>[2x]GSMAEPLKEEDGEDGSAEPPGPVKAEPAHTAASVAAKN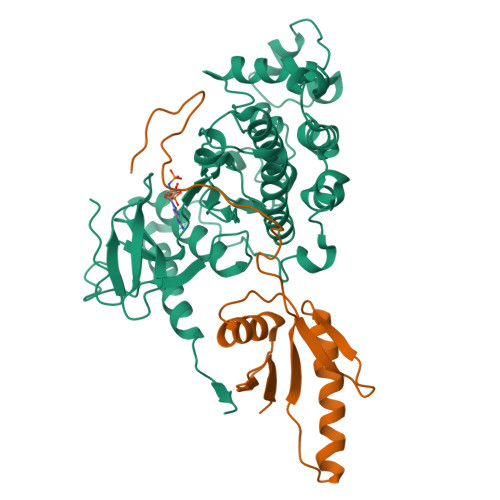LALLKARSFDVTFDVGDEYEIIETIGNGAYGVVSSARRRLTGQQVAIKKIPNAFDVVTNAKRTLRELKILKHFKHDNIIAIKDILRPTVPYGEFKSVYVVLDLMESDLHQIIHSSQPLTLEHVRYFLYQLLRGLKYMHSAQVIHRDLKPSNLLVNENCELKIGDFGMARGLCTSPAEHQYFMTEYVATRWYRAPELMLSLHEYTQAIDLWSVGCIFGEMLARRQLFPGKNYVHQLQLIMMVLGTPSPAVIQAVGAERVRAYIQSLPPRQPVPWETVYPGADRQALSLLGRMLRFEPSARISAAAALRHPFLAKYHDPDDEPDCAPPFDFAFDREALTRERIKEAIVAEIEDFHARREGIRQQIRFQPSLQPVASEPGCPDVEMPSPWAPSGDCAMSGRHHHHHH;>GSVLVIRIKIPNSGAVDWTVHSGPQLLFRDVLDVIGQVLPEATTTAFEYEDEDGDRITVRSDEEMKAMLSYYYSTVMEQQVNGQLIEPLQIFPRACKPPGERNIHGLKVNTRAGPSQSGRHHHHHH[2x]~{N}-[(2-fluorophenyl)methyl]-4-[(4-methylpiperazin-1-yl)methyl]aniline | C19 H24 F N3 | 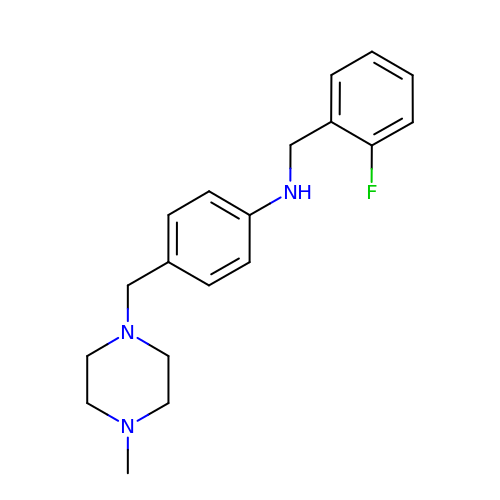GFWGMYAJMIQTFM-UHFFFAOYSA-N> SSKVSEQLKCCSGILKEMFAKKHAAYAWPFYKPVDVEALGLHDYCDIIKHPMDMSTIKSKLEAREYRDAQEFGADVRLMFSNCYKYNPPDHEV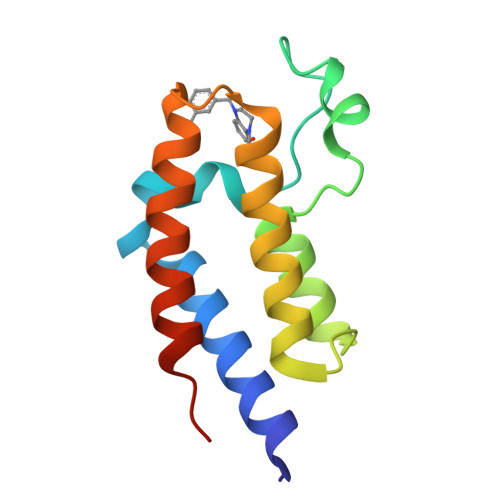VAMARKLQDVFEMRFAKMPDEPEE>[2x]MVLYFIGLGLYDERDITVKGLEIAKKCDYVFAEFYTSLM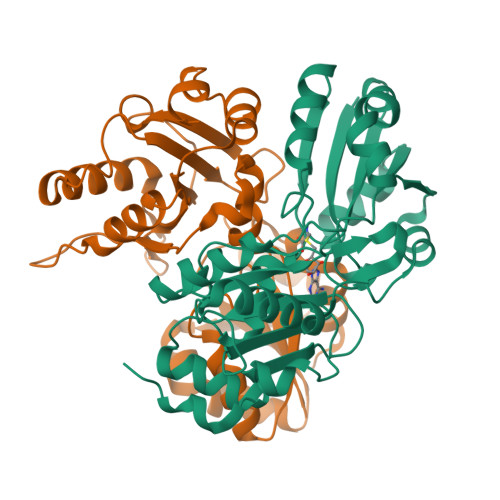AGTTLGRIQKLIGKEIRVLSREDVELNFENIVLPLAKENDVAFLTPGDPLVATTHAELRIRAKRAGVESYVIHAPSIYSAVGITGLHIYKFGKSATVAYPEGNWFPMSYYDVIKENAERGLHTLLFLDIKAEKRMYMTANEAMELLLKVEDMKKGGVFTDDTLVVVLARAGSLNPTIRAGYVKDLIREDFGDPPHILIVPGKLHIVEAEYLVEIAGAPREILRVNV4-methyl-6-[3-(methylamino)prop-1-yn-1-yl]pyridin-2-amine | C10 H13 N3 | 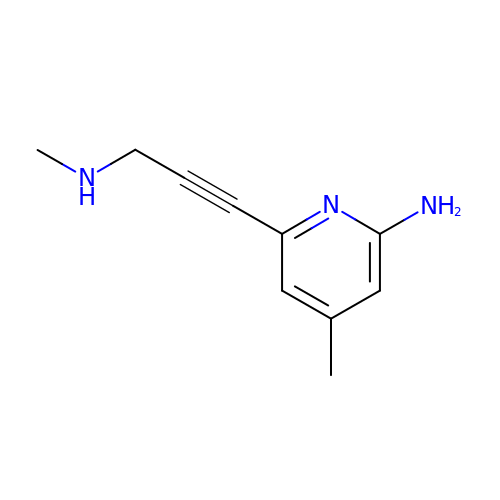NNABKXZKYMQGRR-UHFFFAOYSA-N> MSNYISNYVQSTIVTKTVQNKDKKTGKNSVDPRVINEQLILDAVKQFNQENNKITTENIILQQLRQLQLSFKNILKIQHLQGLERLEKLQLDNNIIEKIENIDHLVNLKWLDLSFNCIKKIEGLDKLKELTDLSLFNNYIEKIEGLHNNTKLNVFSIGNNRLKSYEEITLYFGYKPRGEEGTNDRPEFKRLQVLNVSGNPFTKDKENEYKNHIICAIPNLKYLDYVFIDEGDRQLIRQDEQISNSYNFTTTDYYQQMQAQEQKEEMDRQTLKKKKDARMDILDNLKDEYLKIEDLQRVKIIKPNQINEEIEKYCGKINDHVVEMQAAVIQKHQLILQEMSKTEVSYKEQEALHEKETLQILKEFEHEKKVEFRNWEKEAANGDAKKEESRLKTLLQKTTSLKNKLMDIEIQLVEELEAI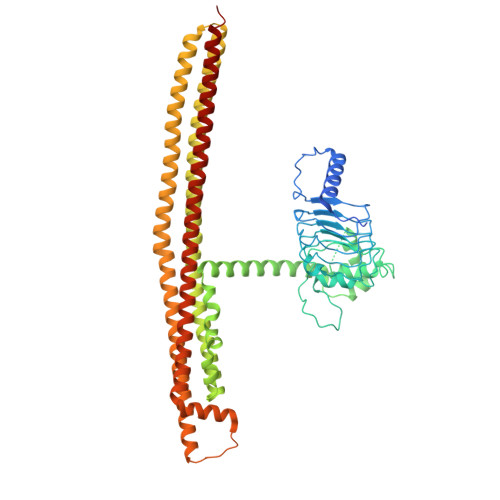FTDYDTKKKETAWKDIEEIIVLGQKKIEEENVKFYSNLNVIKNKEEANYNSTQQQQLEEENNEEDDEKASLLENKEQLAQMIGNIKETLIDSHTKIILSAQMELQKDLAEYAKQQKNKMYERNRKNISQIIAQIDAYQTEINEKLKQGDDESDHEN N-Acetylglucosaminyltransferase-IVa (GnT-IVa, also designated as MGAT4A) forms a β1-4 GlcNAc branch on the α1-3 mannose arm in N-glycans. Downregulation or loss of GnT-IVa causes diabetic phenotypes by dysregulating glucose transporter-2 in pancreatic β-cells. In this study, by combining bioinformatic, biochemical, NMR, molecular dynamics, and crystallographic analyses, we discovered that the GnT-IVa enzyme has a unique lectin domain at its C-terminus, which is critical for its enzymatic reaction. Comprehensive glycan binding assay using 157 glycans and solution NMR reveal that the GnT-IVa lectin domain selectively interacts with the product N-glycans having a β1-4 GlcNAc branch.

Because we could not obtain diffraction-quality crystals of the wild-type lectin domain despite repeated trials, we introduced an alanine mutation at D445, which corresponds to D877 in NagH and is supposed to directly interact with GlcNAc residue. The D445A mutant was successfully purified from bacterial cells and showed no retardation in gel filtration analysis, indicating that the aspartate at position 445 of GnT-IVa also plays a critical role in the sugar binding, as observed in NagH. We successfully obtained well-diffracted crystals of D445A mutant and determined the crystal structure in unliganded form at 1.95 Å resolution. The overall structure of GnT-IVa lectin domain adopts a β-sandwich fold composed of nine β-strands with three short α-helices. Six molecules exist in the asymmetric unit of this crystal. A DALI search revealed that the 3D structure of the GnT-IVa lectin domain shows high structural similarity to those of NagH [PDB code: 2W1U30,] and IFT25/27 complex [PDB code: 2YC431,]. As predicted from sequence analysis, the structural comparison with NagH GlcNAc-containing disaccharide (GlcNAcβ1-3GalNAc) complex demonstrated that amino acid residues that directly interact with the GlcNAc at the non-reducing end in NagH are completely conserved in the GnT-IVa lectin domain. Four residues (Y819, W836, D877, and W935) are completely conserved in GnT-IVa (Y394, W410, D445, and W513). The position of D445A is slightly buried and there is no water molecule corresponding to the hydroxyl group of GlcNAc around D445A. The activity of D445A was reduced to ~62% of that of the wild type, indicating that the glycan binding ability of the lectin domain is required for the efficient enzymatic process.

>GPLGNPPAEVSTSLKVYQGHTLEKTYMGEDFFWAITPTAGDYILFKFDKPVNVESYLFHSGNQEHPGAILLNTTVDVLPLKSDSLEISKETKDKRLEDGYFRIGKFEYGVAEGIVDPGLNPISAFRLSVIQNSAVWAILNEIHIKKVTS[6x]>GMNKAYYIGLMSGTSMDGVDAVLVDFAGEQPQLIGTHTETIPTHLLKGLQRLCLPGTDEINRLGRLDRSVGKLFALAVNNLLAKTKIAKDEIIAIGSHGQTVRHMPNLEVGFTLQIGDPNTIATETGIDVIADFRRKDIALGGQGAPLVPAFHQQTFAQVGKKRVILNIGGIANITYLPGNSEEVLGFDTGPGNTLIDAWVQQVKNESYDKNGAWAASGKTDPQLLAQLLSHPYFSLAYPKSTGRELFNQAWLEQQLSAFNQLNEEDIQSTLLDLTCHSIAQDILKLAQEGELFVCGGGAFNAELMQRLAALLPGYRIDTTSALGVD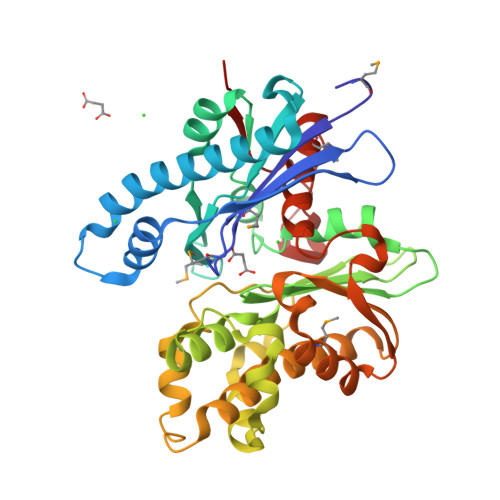PKWAEGIAFAWLAMRYQLGLPANLPAVTGASREAILGGRFSAK[2x]1-[(2R)-4-(9H-pyrido[4',3':4,5]pyrrolo[2,3-d]pyrimidin-4-yl)morpholin-2-yl]methanamine | C14 H16 N6 O | 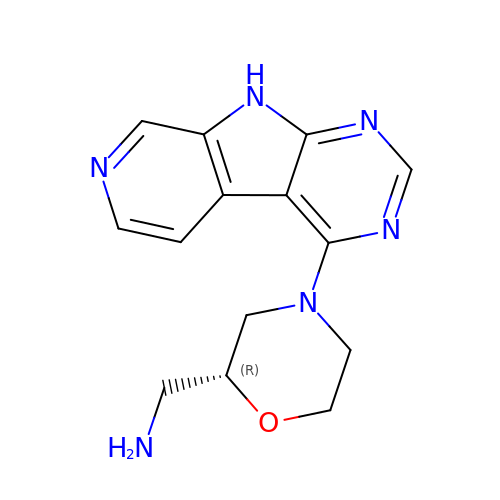ZOMFTMSIQWYIQV-SECBINFHSA-N Here we demonstrate that HSL1 binds IDA/IDL peptides with high, and CLE peptides with lower affinity, respectively. Ligand sensing capability and receptor activation of HSL1 require a SERK co-receptor kinase. Crystal structures with IDA/IDLs or with CLE9 reveal that HSL1-SERK1 complex recognizes the entire IDA/IDL signaling peptide, while only parts of CLE9 are bound to the receptor. Our work reveals that HSL1 is a receptor for IDA/IDL signaling peptides.

The vastly different binding affinities between IDA/IDLs vs. CLE9 to HSL1 prompted us to determine co-crystal structures of four HSL1-IDA/IDL-SERK1 ternary complexes with: IDA, IDL1, IDL2, and IDL3 (at 2.31 Å, 2.38 Å, 2.20 Å, and 2.70 Å, respectively) and the HSL1-CLE9-SERK1 complex at 2.87 Å. In agreement with our biochemical assays, the crystal structures revealed that all IDA/IDL peptides specifically bind to the peptide-binding surface of HSL1. IDA/IDLs adopt a fully extended conformation in the structure. The co-receptor SERK1 interacts with the C-terminal region of the different IDA/IDL peptides (residues 68-69 in IDA), completing the peptide-binding pocket using its N-terminal loop region. Superposition of the four crystal structures yielded an R.M.S.D of ~0.6 Å comparing 590 Cα atom pairs, with IDL peptides perfectly aligning to each other. Our calorimetry experiments reveal that SERK1 binds HSL1 in the presence of IDA/IDL peptides with a dissociation constant (Kd) of around 15 to 50 nM, indicating that IDA/IDLs promote a high-affinity association between HSL1 and the co-receptor SERK1. Taken together, our quantitative binding experiments demonstrate that HSL1 is a bona-fide IDA/IDLs receptor and uses SERK proteins as co-receptor kinases for high-affinity ligand sensing.

> GSSMDNQDGFILQQVKLSLDDPDSYLSSWNSNDASPCRWSGVSCAGDFSSVTSVDLSSANLAGPFPSVICRLSNLAHLSLYNNSINSTLPLNIAACKSLQTLDLSQNLLTGELPQTLADIPTLVHLDLTGNNFSGDIPASFGKFENLEVLSLVYNLLDGTIPPFLGNISTLKMLNLSYNPFSPSRIPPEFGNLTNLEVMWLTECHLVGQIPDSLGQLSKLVDLDLALNDLVGHIPPSLGGLTNVVQIELYNNSLTGEIPPELGNLKSLRLLDASMNQLTGKIPDELCRVPLESLNLYENNLEGELPASIALSPNLYEIRIFGNRLTGGLPKDLGLNSPLRWLDVSENEFSGDLPADLCAKGELEELLIIHNSFSGVIPESLADCRSLTRIRLAYNRFSGSVPTGFWGLPHVNLLELVNNSFSGEISKSIGGASNLSLLILSNNEFTGSLPEEIGSLDNLNQLSASGNKFSGSLPDSLMSLGELGTLDLHGNQFSGELTSGIKSWKKLNELNLADNEFTGKIPDEIGSLSVLNYLDLSGNMFSGKIPVSLQSLKLNQLNLSYNRLSGDLPPSLAKDMYKNSFIGNPGLCGDIKGLCGSENEAKKRGYVLEGSENLYFQ;> GSSMASANLEGDALHTLRVTLVDPNNVLQSWDPTLVNPCTWFHVTCNNENSVIRVDLGNAELSGHLVPELGVLKNLQYLELYSNNITGPIPSNLGNLTNLVSLDLYLNSFSGPIPESLGKLSKLRFLRLNNNSLTGSIPMSLTNITTLQVLDLSNNRLSGSVPDNGSFSLFTPISFANNLDLCGPVTSHPCPLEGSLENLYFQ;> YVPVPASGPSRKHN>[2x]XGQLE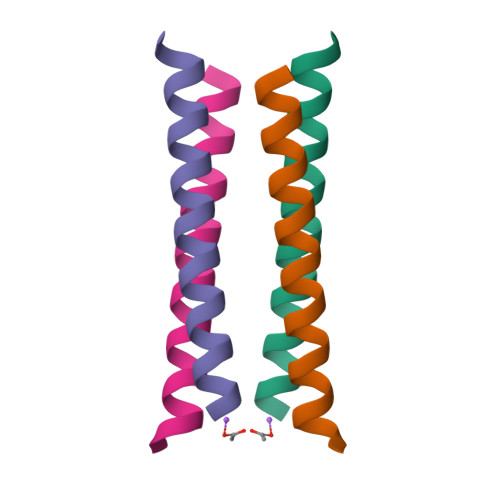EIAQQLEEIAKQLKKIAWQLKKIAQGX>MSEKNVSIVVAASVLSSGIGINGQLPWSISEDLKFFSKITNNKCDSNKKNALIMGRKTWDSIGRRPLKNRIIVVISSSLPQDEADPNVVVFRNLEDSIENLMNDDSIENIFVCGGESIYRDALKDNFVDRIYLTRVALEDIEFDTYFPEIPETFLPVYMSQTFCTKNISYDFMIFEKQEKKTLQNCDPARGQLKSIDDTVDLLGEIFGIRKMGNRHKFPKEEIYNTPSIRFGREHYEFQYLDLLSRVLENGAYRENRTGISTYSIFGQMMRFDMRESFPLLTTKKVAIRSIFEELIWFIKGDTNGNHLIEKKVYIWSGNGSKEYLERIGLGHREENDLGPIYGFQWRHYNGEYKTMHDDYTGVGVDQLAKLIETLKNNPKDRRHILTAWNPSALSQMALPPCHVLSQYYVTNDNCLSCNLYQRSCDLGLGSPFNIASYAILTMMLAQVCGYEPGELAIFIGDAHIYENHLTQLKEQLSRTPRPFPQL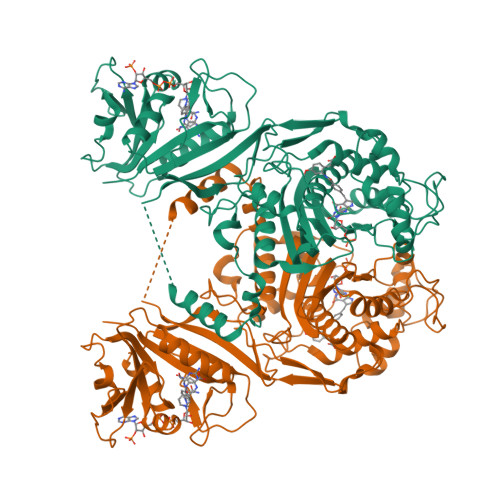KFKRKVENIEDFKWEDIELIGYYPYPTIKMDMAV[5x]6-amino-5-{[(3S)-4,4-difluoro-1-{[4-(trifluoromethoxy)phenyl]acetyl}pyrrolidin-3-yl]oxy}-N-methylpyridine-3-carboxamide | C20 H19 F5 N4 O4 | 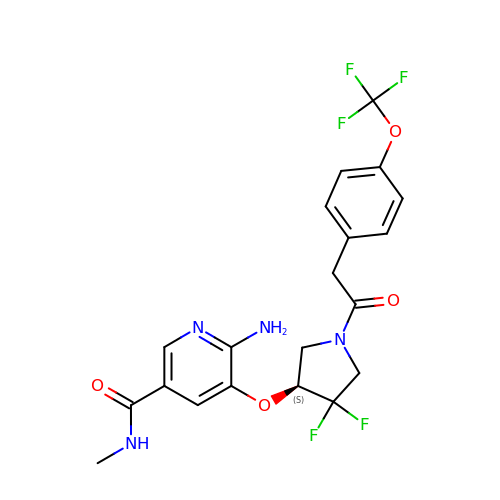FTAFQADCGCSJAH-HNNXBMFYSA-N> MKEKIRKKILLAPEEPGVYIFKNKGVPIFIGKAKRLSNRLRSYLNPQ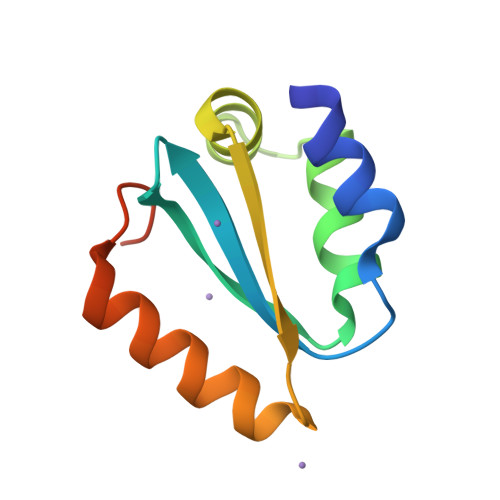TEKVFRIGEEADELETIVVMNEREAFILEANLIKKYRPKYNVRLKDTDF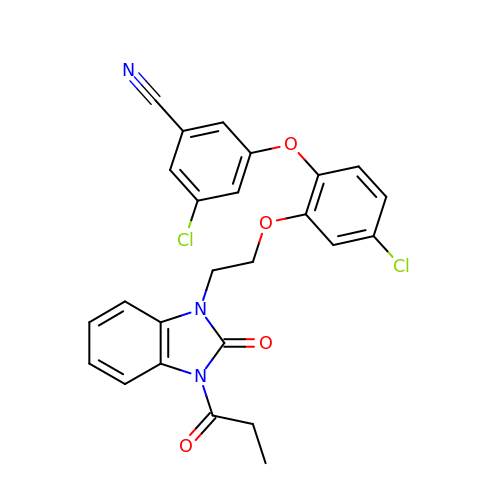3-chloro-5-{4-chloro-2-[2-(2-oxo-3-propanoyl-2,3-dihydro-1H-benzimidazol-1-yl)ethoxy]phenoxy}benzonitrile | C25 H19 Cl2 N3 O4 | LGSPOOOHYUJKNO-UHFFFAOYSA-N3-(2-hydroxyethyl)-2,2-bis(hydroxymethyl)pentane-1,5-diol 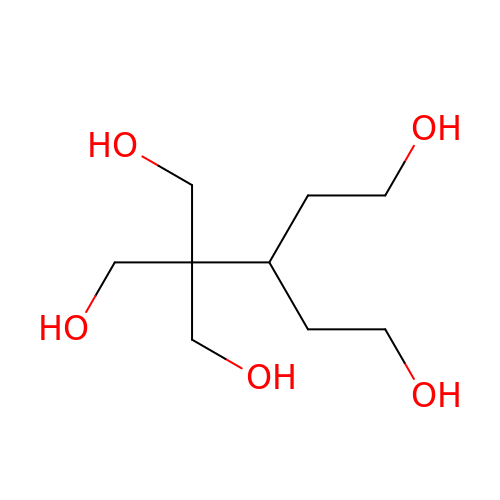| C9 H20 O5 | SBDIPIUGTYTDCJ-UHFFFAOYSA-N3-(1,3-benzodioxol-5-yl)propanoic 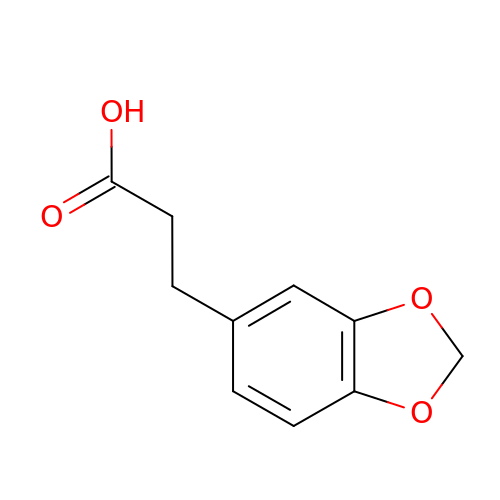acid | C10 H10 O4 | UIYJGLLTSVRSBM-UHFFFAOYSA-N>GDADVLVKWSEDLANLPSID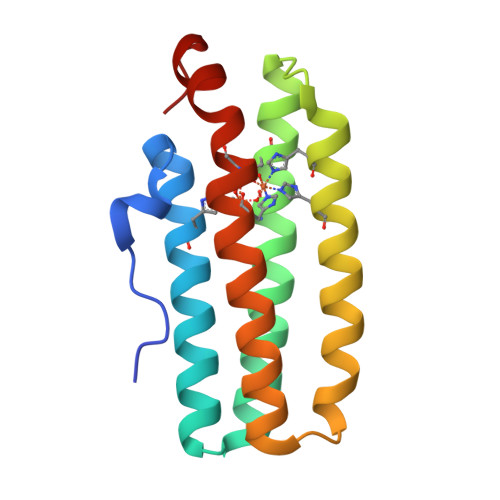TQHKRLVDYINDLYRAARRRDMDKAREVFDALKNYAVEHFGYEERLFADYAYPEATRHKEIHRRFVETVLKWEKQLAAGDPEVVMTTLRGLVDWLVNHIMKEDKKYEAYLRERGVS[2x]> MVNTEEDGLPRLIDAIEEASKIPAKRRQTPIKPTIEKLTTHLYTHGASPDSLLRLADLLTLRNHLDQASLAAITRNLYPSSTVSDEVVLRFIGALGHGQLKPTLALQALFLRWLVMVYHLLENPGVLGQVYGVLFDLLDTAAIRPQLCHLLALVTRRKHVRPFRIQAILTLSRQTGGDPNLTGLLRVFKNYYPEIIVGDATKGRASAFKHPDPQWRQHLDEIQQRRSEA

As the core subunits of the CCAN, CENP-H, CENP-I and CENP-K (also known as Mcm16/Ctf3/Mcm22 in Saccharomyces cerevisiae and Fta3/Mis6/Sim4 in Schizosaccharomyces pombe) assemble into a ternary complex and are essential for the integrity of the kinetochore. At the inner layer, a number of centromere proteins form a network termed CCAN (the constitutive centromere-associated network) that binds to the centromere throughout the cell cycle. We here determined the crystal structures of CENP-I N-terminus alone from Chaetomium thermophilum and its complex with CENP-H/K from Thielavia terrestris, and verified the identified interactions. CENP-I integrates into the CENP-H/K complex by binding to the C-terminus of CENP-H, leading to formation of the ternary complex in which CENP-H is sandwiched between CENP-K and CENP-I. Our sequence comparisons and mutational analyses showed that this architecture of the CENP–H/I/K complex is conserved in human.

Instead, we found that CENP-I from another fungi C. thermophilum (ct) is 62% identical in sequence to thCENP-I, and showed excellent biochemical behavior. Due to the high degree of sequence similarity, we tested whether ctCENP-I could form a hybrid complex with thCENP-H/K for crystallization. It has been shown that the N-terminal region of hsCENP-I is necessary and sufficient for interacting with hsCENP-H/K. We therefore purified the corresponding N-terminal region of ctCENP-I (ctCENP-INT), which indeed formed a stable hybrid complex with the thCENP-H/K proteins. We first determined the structure of ctCENP-INT at 2.3Å with the Single-wavelength Anomalous Dispersion (SAD) method. ctCENP-INT adopts the HEAT repeat fold containing five pairs of helixes α1–α10. A following helix α11 folds back and packs against the HEAT repeat with extensive hydrophobic interactions, which likely contributes to the protein stability. The structure of ctCENP-I is similar to a model of hsCENP-I proposed previously, except that helix α11 packs on the surface of the HEAT repeat in our structure. The structure of ctCENP-INT in the complex is very similar to the apo state.>[8x]ASWSHPQFEKIEGRRDRGPEFLAKQY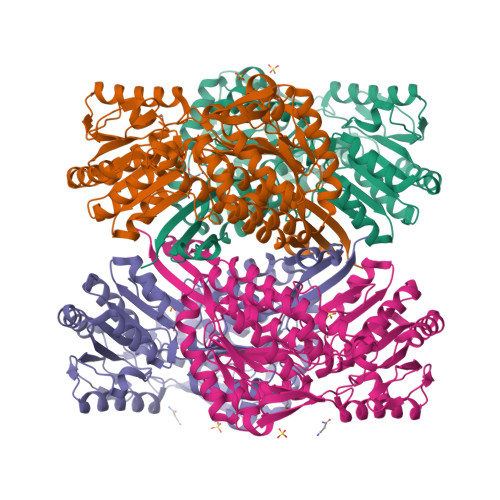KNLVNGEWKLSENEITIYAPATGEELGSVPAMTQAEVDAVYASAKKALSDWRTLSYVERAAYLHKAADILVRDAEKIGAILSKEVAKGHKAAVSEVIRTAEIINYAAEEGLRMEGEVLEGGSFEAASKKKIAIVRREPVGLVLAISPFNYPVNLAGSKIAPALIAGNVVALKPPTQGSISGLLLAEAFAEAGIPAGVFNTITGRGSVIGDYIVEHEAVNFINFTGSTPIGEGIGKLAGMRPIMLELGGKDSAIVLEDADLALAAKNIVAGAFGYSGQRSTAVKRVLVMDKVADQLAAEIKTLVEKLSVGMPEDDADITPLIDTSAADFVEGLIKDATDKGATALTAFNREGNLISPVLFDHVTTDMRLAWEEPFGPVLPIIRVTTVEEAIKISNESEYGLQASIFTTNFPKAFGIAEQLEVGTVHLNNKTQRGTDNFPFLGAKKSGAGVQGVKYSIEAMTTVKSVVFDIQ Complex III (CIII2), also called the cytochrome bc1 complex or ubiquinol-cytochrome c oxidoreductase, is an obligate dimer that transfers electrons from ubiquinol in the IMM (reduced by CI, CII, or alternative NADH dehydrogenases) to soluble cytochrome c in the intermembrane space (IMS). Complex IV (CIV), also called cytochrome c oxidase, transfers electrons from cyt c to molecular oxygen, reducing it to water. In the IMM, respiratory complexes can be found as separate entities or as higher-order assemblies known as supercomplexes. Here we present the cryoEM structures of CIII2 and SC III2+IV from the vascular plant Vigna radiata (mung bean) at nominal resolutions of 3.2 Å and 3.8 Å, respectively.

The V. radiata (Vr) structure confirms that VrCIII2 contains 10 subunits per CIII monomer (three conserved, mitochondrially encoded subunits and seven accessory subunits), similar to yeast and mammals. The MPP domain, composed of two MPP-α/β heterodimers (one per CIII protomer), extends into the matrix. Consistent with their known flexibility and conformational heterogeneity, the linker and head domains of UCR1 (Rieske iron-sulfur subunit) were disordered in our reconstruction and an atomic model was not produced for this region of UCR1. All heme groups (heme bH, bL and heme c1) were clearly visible and modelled into each cyt b and cyt c1 subunit of the dimer. A catalytic Zn2+ ion was also visible and modelled into each MPP-β subunit. Our cryoEM map shows density for the Zn2+ ion, which is coordinated by residues His137, His141, Glu217. Density consistent with cardiolipin, phosphatidylethanolamine and phosphatidylcholine lipids was found and modelled into the VrCIII2 map. Nevertheless, no clear density for endogenous quinone was visible in any of the binding sites of the V. radiata dimer. Thirdly, a ~ 50 amino-acid N-terminal extension on VrMPP-β folds into an alpha helix that forms extensive contacts with MPP-α of the same CIII protomer as well as with VrQCR7 of the opposite protomer. The largest variability component revealed a near-continuous conformational motion in the position of the head domain of UCR1, demonstrating its swinging motion from the proximal b position (close to COB’s QP-site) to its distal c position (close to CYC1) during the Q-cycle (Xia et al., 2013; Cooley, 2013; Berry and Huang, 2011).

>[2x]MSLNRLLSAARRSDRRASALSSFRSLSASPALAPSAASPPAPPPPTAMIYDRAAEAIKSKLRQLENPDPRFLKHGNPRPALSDHTRILAAPETRVTTLPNGLRVATESSLAARTATVGVWIDAGSRFETEETNGTAHFLEHMIFKGTERRNARELEEEIENMGGHLNAYTSREQTTYYAKVTDSDVPQALDILADILQNSRFEENRISRERDVILREMEEVEGQTEEVIFDHLHATAFQYTPLGRTILGPAQNIKTITKAHLQSYIQTHYTAPRMVIAASGAVKHEDIVEQVKKLFTKLSTDATTTAQLVAKEPAIFTGSEVRMLDDDIPLAQFAVAFEGASWKDPDSIALMVMQAMLGSWNKTAGGGKHMGSELAQRVGINEVAESIMAFNTNYKDTGLFGVYAVAKPDCLDDLSYAIMQETTKLVYRVSEDDVTRACNQLKSSLLLHIDGTSPVAEDIGRQLLTYGRRIPFAELFARIDAVDASTIKRVANRFIYDKDVAIAAMGPIQRLPDYNWFRRRTYWNRY;>[2x]MYRAAASSFRRHLKGHGSKLGSTRSSTSAAVAARTSKGGLFSWLTGERSSSLPSLDIPLGGVVLPDPLPDSVEQSKTKITTLSNGLKIASETSPNPAASIGLYLDCGSIYETPFSSGASHLLERMAFKSTTNRSHFRIVREVEAIGGNIGASASREQMGYTFDALKTYVPQMVELLVDCVRNPAFLDWEVNEELRKVKAELGELSNNPQGLLLEAIHSAGYSGALAYPLLAPEAALNRLDGPSLEEFVAENYTAPRMVLAAAGVEHEELVSIAEPLLSDLPNVPRPDEPKSVYVGGDFRRHGESGGTHVALAFEVPGGWHKEKDAIVLTVLQMLMGGGGSFSAGGPGKGMHSRLYLRVLNEYQQIQSFSAFNSIFNNTGLFGIYASTSPDFAPKAVDIAAKELIAIASPGQVTQVQLDRAKKSTKSAVLMNLESRMIASEDIGRQILTYGERKPLEQFLKAVDEITLNDITKISQKIISSPLTMASYGDVLSVPSYESVNRKFHAK;>MTIRNQRFSLLKEPISSTLNQHLIDYPTPSNLSYWWGFGSLAGICLVIQIVTGVFLAMHYTPHVDLAFNSVEHVMRDVEGGWLLRYMHANGASMFFIVVYLHIFRGLYYASYSSPREFVWCLGVVIFLLMIVTAFTGYVLPWGQMSFWGATVITSLASAIPVVGDTIVTWLWGGFSVDNATLNRFFSLHYLLPFLLVGASLLHLAALHQYGSNNPLGVHSEMDQISFYPYFYVKDLVGWVAFAIFFSIWIFYAPNVLGHPDNYIPANPMSTPPHIVPEWYFLPIYAILRSIPDKSGGVAAIALVFICLLALPFFKSMYVRSSSFRPIYQGIFWLLLADCLLLGWIGCQPVEAPFVTIGQISSFVFFLFFAITPILGRVGRGIPNSYTTDETEM[2x];>[2x]MTGGVFQLLRRKLHPQFTNSSLLSPIIAKKDGAGSTGSRSLKVLALIGAGVSGFFSFSTVAVADEAEHGLACPSYPWPHKGILSSYDHASIRRGHQVYTEVCASCHSMSLISYRDLVGVAYTEEEVKAMAAEIEVVDGPNDEGEMFTRPGKLSDRFPQPYANEAAARFANGGAYPPDLSLITKARHNGQNYVFSLLTGYRDPPAGVSIREGLHYNPYFPGGAIAMPKMLNDGAVEYEDGTPATEAQMGKDVVSFLSWAAEPEMEERKLMGFKWIFVLSLALLQAAYYRRLRWSVLKSRKLVLDVVN;>[2x]MLRVAAKRLSSLSSSAWRANHAASAVLSRNPVAPSLSTEEHRSDPFSLRPEFFLPIRGYATDSLFHPKENSLIPEIPATVAAVKNPSSKIIYDEHNHERFPPGDPSKRAFAYFVLTGGRFVYASLIRLLVLKFVLSMSASKDVLALASLEVDLSSIEPGTTVTVKWRGKPVFIRRRTEDDIKLANSVDVASLRDPQQDAERVKNPEWLIVIGVCTHLGCIPLPNAGDFGGWFCPCHGSHYDISGRIRKGPAPYNLEVPTYTFLEENKLMIG;>[2x]MASFLQSFLDPKKNWLAAQHMKSLVKRLSKYGLRYDDLYDPYYDLDVKEALNRLPKEVVDARHARLKRAIDLSMKHEYLPEDLQAMQTPFRGYLQDMLALVKRERAEREALGGLPLYQRSIP;>[2x]MGKQIVPVKSVIYALSPFQQKVMTGLWKDLPTKIHHKVSENWISATLLLGPLVGTYAYVQNYLEKEKLHHRY;>[2x]MADEEPVDQKRYLEESCKPKCVKPLLEYQACIKRIHGDDSGQKHCTGQYFDYWFCVDKCVAPKLFTKLK;>METVARRRGGGIFESLYKVVMRRNSVYVTFVIAGAFLGERAVDYGIHKLWEANNVGKRYEDIPVLGQKLSEE[2x];>[2x]MAGLPARLRIQPADVKAAAMWGVAAATGGLYLVQVSILVLPPVKVVFHFYLVSGFRICLDVKDLRTMPCSAPRIWRLYILI>[2x]CGCGAATTCGCG

The rational design of small molecules that target specific DNA sequences is a promising strategy to modulate gene expression. This report focuses on a diamidinobenzimidazole compound, whose selective binding to the minor groove of AT DNA sequences holds broad significance in the molecular recognition of AT-rich human promoter sequences. The specialized method of X-ray crystallography was utilized to investigate how the sequence-dependent recognition properties in general, A-tract, and alternating AT sequences affect the binding of diamidinobenzimidazole in the DNA minor groove. A strong and direct hydrogen bond between the N-H of the benzimidazole and an H-bond acceptor atom in the minor groove is essential for DNA recognition in all sequences described. In addition, the diamidine compound specifically utilizes an interfacial water molecule for its DNA binding.

The AATT-DB1476 complex structure reveals a unique 1:1 binding mode with two orientations of DB1476 observed in the minor groove. The electron density map of AATT-DB1476-I and AATT-DB1476-II does not show an unequivocal orientation assignment. Thus, we presented a structure with two possible ligand orientations. The ligand in the structures AATT-DB1476-I and AATT-DB1476-II utilizes an interfacial water molecule at one amidine end to bind to the DNA. AATT-DB1476-I and AATT-DB1476-II show identical interactions with the DNA bases at the minor groove. The BI-N-H in both complexes forms a strong direct H-bond in a bifurcated manner with the O2s of T7 and T19, respectively. In addition to the strong BI-N-H hydrogen bonds, one of the amidines in each complex, A-N6 in AATT-DB1476-I and C-N4 in AATT-DN1476-II, forms a strong direct hydrogen bond with O2 of C9. In the X-ray structure of AATT-DB1476-I, the C-N4 of the DB1476 uses an interfacial water molecule to form a hydrogen bond with the O2 of T20 (−NH•••O – H•••O=T). In the AATT-DB1476-I complex, the amidine group (N5/N6) at Ph-amidine (A) forms a strong direct H-bond with O2 of C21 (C21=O---N5/N6, 2.8 Å) for more than 91% of the time and for the remainder of the time, N5/N6 amidine uses interfacial water to connect with the C21 base. The N3/N4 amidine needs interfacial water for approximately 70% of the time to connect with O2 of T8 (T8 = O---H-O----N4/N3, with average bond distances 2.9, 3.0 Å, respectively).>ILPDSVDWREKGCVTEVKYQGSCGASWAFSAVGALEAQLKLKTGKLVSLSAQNLVDCSTEKYGNKGCNGGFMTTAFQYIIDNKGIDSDASYPYKAMDQKCQYDSKYRAATCSKYTELPYGREDVLKEAVANKGPVSVGVDARHPSFFLYRSGVYYEPSCTQNVNHGVLVVGYGD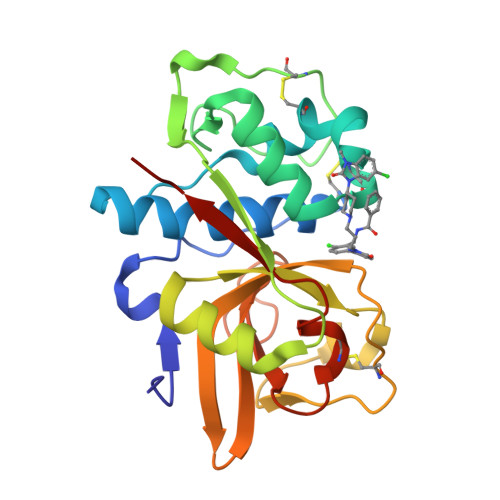LNGKEYWLVKNSWGHNFGEEGYIRMARNKGNHCGIASFPSYPEILQGGG[2x]> GPGSEFEENEDSDPLPDNWEMAYTEKGEVYFIDHNTKTTSWLDPRLAKKAKPPEECKENELPYGWEKIDDPIYGTYYVDHINRRTQFENPVLEAK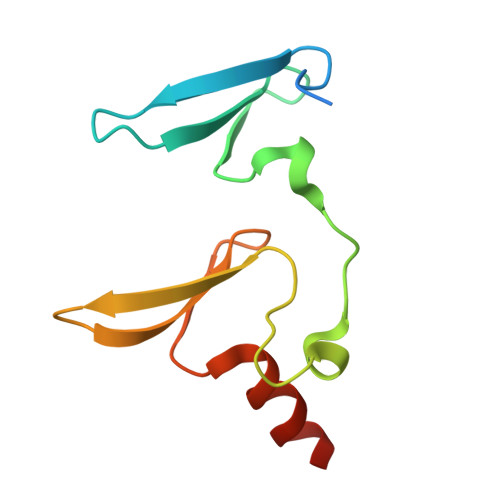RKLQQHN>[8x]MAKKTSSKGKLPPGPTPLPFIGNYLQLNTEQMYNSLMKISERYGPVFTIHLGPRRVVVLCGHDAVKEALVDQAEEFSGRGEQATFDWLFKGYGVAFSNGERAKQLRRFSIATLRGFGVGKRGIEERIQEEA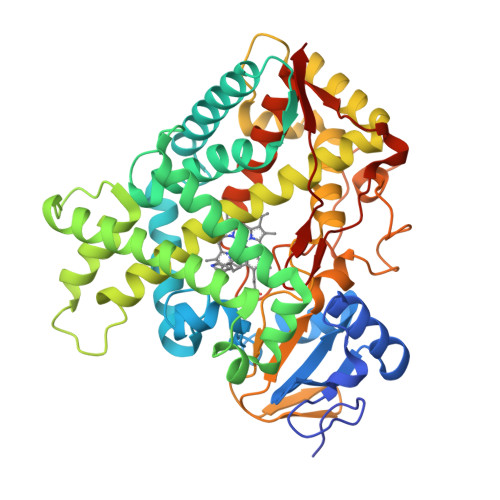GFLIDALRGTHGANIDPTFFLSRTVSNVISSIVFGDRFDYEDKEFLSLLRMMLGSFQFTATSTGQLYEMFSSVMKHLPGPQQQAFKELQGLEDFIAKKVEHNQRTLDPNSPRDFIDSFLIRMQEEEKNPNTEFYLKNLVMTTLNLFFAGTETVSTTLRYGFLLLMKHPEVEAKVHEEIDRVIGKNRQPKFEDRAKMPYTEAVIHEIQRFGDMLPMGLAHRVNKDTKFRDFFLPKGTEVFPMLGSVLRDPRFFSNPRDFNPQHFLDKKGQFKKSDAFVPFSIGKRYCFGEGLARMELFLFFTTIMQNFRFKSPQSPKDIDVSPKHVGFATIPRNYTMSFLPRHHHH> QGPTSIWTKGVTPPTNFIEGTDGSHAPYIANQGWYDITKTFNGKDDLLSAAATAGNMLHWWFDQNKNQIEGYLTEHPEKQAIIFNGEQMFDVKEAISTKDRQLDSKLFEYFKEKAFPTLSARRRGVFPDHVIDMFINGYRLSLDNYDKTPVKEGNKDLRGGIFDQVFTRGDQSKLLTNRYNLRTKTINEISQLIKQELIAGKALAISHTYNNIGISHVINLWGADFNSEGNLEAIYVTDSDSNASIGMKKYYVGVNSAGEVAVSSKKIDSEHLGAAALGLYTLSAGQGIWH

In this work, we describe a novel protease of S. canis, termed IdeC (Immunoglobulin G degrading enzyme of S. canis), which may be involved in bacterial immune evasion. We demonstrated IdeC is a cysteine protease that cleaves feline, canine, and human IgG between the hinge and CH2 regions, defining a new virulence determinant for S. canis. The structure of IdeC presents the α/β fold characteristic of the papain superfamily of cysteine proteases, consisting of an α-helix followed by an antiparallel β-sheet comprised of four/five β-strands. The active site, the canonical catalytic triad for papain-like cysteine peptidases (Cys-His-Asn/Gln/Asp/Glu), is situated at the interface and involves residues from both domains.

To enhance crystal quality, a truncated form of the inactive IdeC was produced in which the first 48 residues were removed (IdeC_T48_C94S). Crystallization experiments with the truncated IdeC produced new crystals in the cubic P 21 3 space group that allowed the structural determination of this variant at 2.25 Å resolution. Comparison with the IdeC_C94S structure revealed a high degree of similarity (rmsd of 0.376 Å for 229 Ca atoms superimposition), although notable differences were located at the PBL loop, further closing the cavity and blocking the substrate binding site in the IdeC_C94S_T48 structure. No sulfate ion was found in the IdeC_C94S_T48 active site, which may account for the different conformations of the PBL. In the IdeC_C94S_T48 structure, the PBL is stabilized by polar interactions involving the main chains of His253, Tyr255, Ile260, His262, Ala320, and Ala321, as well as with the side chains of Thr254, Tyr244, and His262. Additional structural differences between both structures were noted in loops 63–69, 186–194, 226–231, 301–304, and 309–323 and in residues 125–137, which form a small β-sheet (β−3 and β−4) in the truncated IdeC structure. Minor changes were observed between residues 86–89, 160–163, and in α−2. Similarly, we conducted crystallographic experiments with the truncated form of IdeC and the IgG-Fc. Unfortunately, only crystals of IdeC alone were obtained.> STKHILDD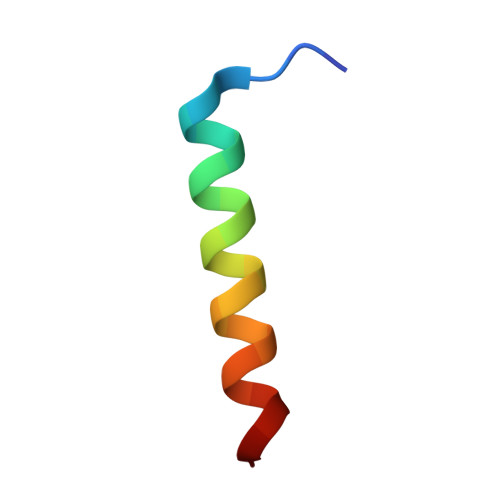ISTMFDALADQLDAMLD>MAFAPIPRITWEHREVHLVQFHEPDIYNYSALLLSEDKDTLYIGAREAVFAVNALNISEKQHEVYWKVSEDKKAKCAEKGKSKQTECLNYIRVLQPLSATSLYVCGTNAFQPACDHLNLTSFKFLGKNEDGKGRCPFDPAHSYTSVMVDGELYSGTSYNFLGSEPIISRNSSHSPLRTEYAIPWLNEPSFVFADVIRKSPDSPDGEDDRVYFFFTEVSVEYEFVFRVLIPRIARVCKGDQGGLRTLQKKWTSFLKARLICSRPDSGLVFNVLRDVFVLRSPGLKVPVFYALFTPQLNNVGLSAVCAYNLSTAEEVFSHGKYMQSTTVEQSHTKWVRYNGPVPKPRPGACIDSEARAANYTSSLNLPDKTLQFVKDHPLMDDSVTPIDNRPRLIKKDVNYTQIVVDRTQALDGTVYDVMFVSTDRGALHKAISLEHAVHIIEETQLFQDFEPVQTLLLSSKKGNRFVYAGSNSGVVQAPLAFCGKHGTCEDCVLARDPYCAWSPPTATCVALHQTESPSRGLIQEMSGDASV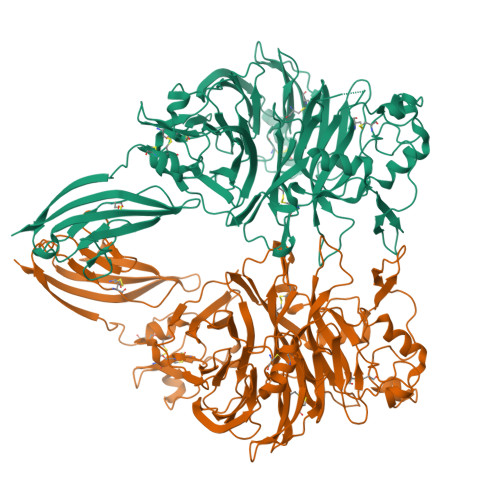CPDKSKGSYRQHFFKHGGTAELKCSQKSNLARVFWKFQNGVLKAESPKYGLMGRKNLLIFNLSEGDSGVYQCLSEERVKNKTVFQVVAKHVLEVKVVPKPVVAPTLSVVQTEGSRIATKVLVASTKHHHHHH[2x]> XVEPI;> VVGGTEAQRNSWPSQISLQYRSGSSWAHT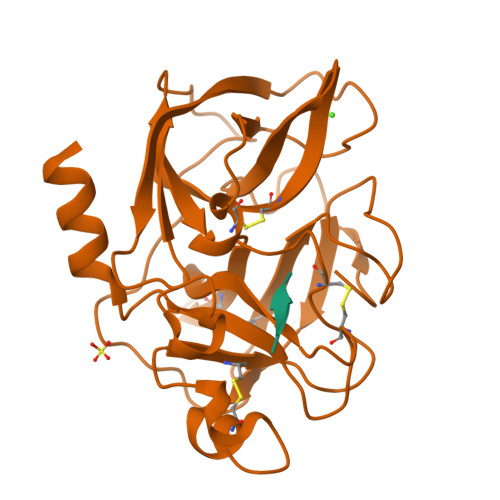CGGTLIRQNWVMTAAHCVDRELTFRVVVGEHNLNQNNGTEQYVGVQKIVVHPYWNTDDVAAGYDIALLRLAQSVTLNSYVQLGVLPRAGTILANNSPCYITGWGLTRTNGQLAQTLQQAYLPTVDYAICSSSSYWGSTVKNSMVCAGGDGVRSGCQGDSGGPLHCLVNGQYAVHGVTSFVSRLGCNVTRKPTVFTRVSAYISWINNVIASN> MMFLPTDYCCRLSDQEYMELVFENGQILAKGQRSNVSLHNQRTKSIMDLYEAEYNEDFMKSIIHGGGGAITNLGDTQVVPQSHVAAAHETNMLESNKHVDDSETLKASSSKRMMVDYHNRKKIKFIPPDE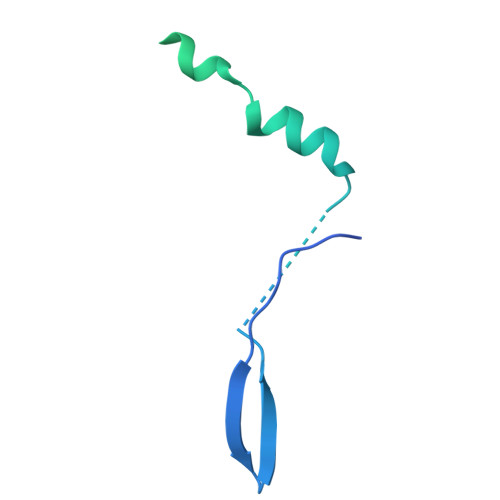QSVVADRSFKLGFDTSSVGFTEDSEGSMYLSSSLDDESDDARPQVPARTRK In the methanogenic pathway from H2 and CO2, the membrane-spanning methyl-tetrahydromethanopterin (CH3-H4MPT):coenzyme M (CoM-SH) methyltransferase complex (MtrA–H) catalyses the exergonic methyl transfer from CH3-H4MPT to CoM-SH (ΔG°′ = −30 kJ/mol) coupled with endergonic sodium-ion gradient formation. The only prosthetic group required for catalysis is vitamin B12 (cobalamin) bound to MtrA. Here, we report on the X-ray structures of the B12-binding domain of membrane-associated MtrA from Methanocaldococcus jannaschii and of the MtrA homologue from M. fervidus in complex with cobalamin. Analyses of these structures reveal a cobalamin-binding site that differs from other B12-binding proteins in an unexpected manner and also provides initial hints of how the energy of cobalt demethylation is transformed into conformational energy used for the ultimate sodium-ion translocation process.

Primary structure analysis predicts MtrC, MtrD and MtrE as integral membrane proteins with at least six transmembrane helices, MtrA, MtrB, MtrF and MtrG as peripheral proteins with one transmembrane helix anchor, and MtrH as a peripheral protein without a membrane anchor. Membrane-associated MtrA devoid of the C-terminal transmembrane helix was over-produced in Escherichia coli 20 years ago in a soluble but cobalamin-free form, and the holoenzyme was reconstituted by unfolding and refolding in the presence of cobalamin11. However, cobalamin appears to bind less tightly to isolated MtrA than to MtrA in the MtrA–H complex. The structure of cytoplasmic MtrA complexed with cobalamin and the structure of the soluble domain of MtrA without cobalamin were essentially identical. This finding suggested that the MtrA structures observed in this work were relaxed forms.

> SHMANKREPAPGWPIVSGEYVVGNPESCVGVVTLGSHGLEQACIDAGAAIAGPCHTENLGIEKVVANYISNPNIRFMILCGSEVQGHITGQCFKALWENGIGDDGGIIGAKGAIPFLENVNKEAVERFRRQIVEVVDLIDCEDIGKITQAIKECLSKDPGAIDEDPFIIELE;> GSHMANKREPAPGWPIVSGEYVVGNPESCVGVVTLGSHGLEQACIDAGAAIAGPCHTENLGIEKVVANYISNPNIRFMILCGSEVQGHITGQCFKALWENGIGDDGGIIGAKGAIPFLENVNKEAVERFRRQIVEVVDLIDCEDIGKITQAIKECLSKDPGAIDEDPFIIELE> GPLGSGRPSLGFTLDLHRIQRDYIDLVPKHWHVISLSLSDGGHDLCITRLQAGQAPFVLRLPLERASSRDSSVDETDVFDFHTGRAELLEIIKEINRTCHDSRDMAA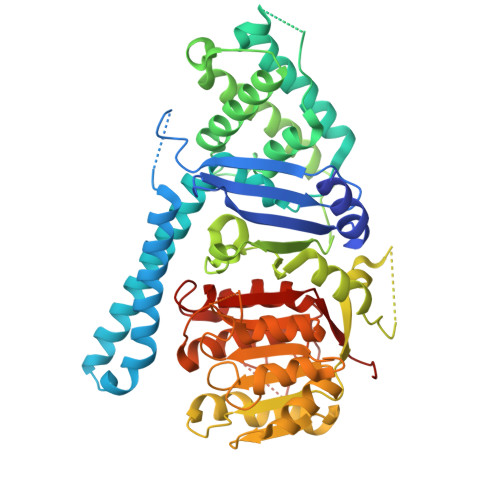KGEREKWWAEREALDQRLKELLMNIEHVWLGGFRGVFSQHGRRPELLEKFRAMFEGVLDKHLPSRRQVGRGKKGKGVAGQTKVVLDGNVLELFIGLGDATKSGADFDEELTDLLYFVVDILQFHGERNAYDEIDFDSMVVETMDALMAYHAEANAAPESDSHAHTILVLDKQLHVFPWESLPCLQGLAVSRIPSLACLRKLLLDRRRSSSQIQGEDSEEEDPRSAGHHAPLSGGTYILNPSSDLLSTQKTFESLFSTHLHSPNSWTRIISRPPTEPEFLSALTHSPILLYFGHGSGAQYIRSRNIRHLDHCRATVLLMGCSSAALTAKGEFEPSGPVWNYMLAGAPAVVGTLWDVTDRDIDRFAGGVLEGWGVLPEGCMGEKNGKKKAGRNGLSLVQAVAKARDRCRFRYVTAAAAVVYGIPVYVDVDGKSKD> MKLSPREIEKLGLHNAGYLAQKRLARGLRLNYTEAVALIATQIMEFVRDGDKTVAQLMSIGRELLGRRQVLPAVPKLVESVQVEATFPDGTELVTIHDPIACENGNLELALLGSFLPVPSLDKFTANDEDNRIPGEIIVVGGNLVLNDGRKAVILKVVNNGDRPVQVGSHYHFIELNPYLTFDRRKAYGMRLNIAAGNASRFEPGECKEVLLVSIGGNKVIRGGNAIADGPVNASNCIAAMQAVITRGFGHVEEANAAEGQTG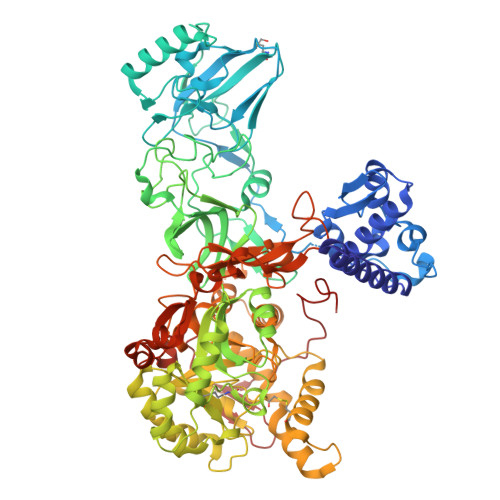EDASCPFTTVISREEYANKYGPTTGDKIRLGDTALFAEIEKDFAIYGDECTFGGGKVIRDGMGQSCGHPPALSLDTVITNAVIIDYSGIIKADIGIKDGLIHSIGKSGNPDVMDGVFQNMTTGVNTEVIAGEGLIVTAGAIDCHVHYICPQLVYEAVTSGITTLVGGGTGPTAGTRATTCTPAPIQMKLMLQSTDDLPLNFGFTGKGNCAKPDELHEIIKAGAMGLKLHEDWGTTPAAIDSCLTIAEQYDIQVNIHTDTLNESGFVEHTIAAFKGRTIHTYHSEGAGGGHAPDIIKVCGEKNVLPSSTNPTRPLTSNTIDEHVDMLMVCHHLDANIAEDVAFSASRIREATIAAEDILHDMGAISIISSDSQAMGRIGEVISRTWQTADKMKSARGPLQPGEEANDNFRIKRYVAKYTINPAIANGFSQYVGSVEVGKLADLVMWKPSFFGAKPEMVIKGGEVAYANMGDPNASIPTPEPVKMRPMYGALGKAGGALSIAFVSKAALDQRVKVLYGLNKRVEAVSNVRKLTKLDMKLNDALPAITVDPDSYTVTADGVVLTCFVATTVPLSRNYFIF>SNAMIKQRTLKNIIRATGVGLHSGEKVYLTLKPAPVDTGIVFSRTDLDPVVEIPARAENVGETTMSTTLVKGDVKVDTVEHLLSAMAGLGIDNAYVELSASEVPIMDGSAGPFVFLIQSAGLQ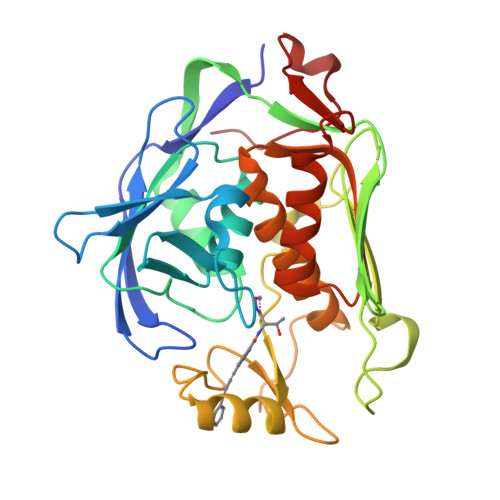EQEAAKKFIRIKREVSVEEGDKRAVFVPFDGFKVSFEIDFDHPVFRGRTQQASVDFSSTSFVKEVSRARTFGFMRDIEYLRSQNLALGGSVENAIVVDENRVLNEDGLRYEDEFVKHKILDAIGDLYLLGNSLIGEFRGFKSGHALNNQLLRTLIADKDAWEVVTFEDARTAPISYMRP[4x]>AETDVLIVGAGPAGAMSATLLASLGIRSLMINRWRSTSPGPRSHIINQRTMEILRDIGLEESAKSLAVPKEYMGEHVYATSLAGEEFGRIPAWASHPQAHAEHELASPSRYCDLPQLYFEPMVVSEAALRGADVRFLTEYLGHVEDQDGVTARLLDHVSGAEYEVRAKYIIGADGAHSLVAQNAGLPFEGQMGIGDSGSINIEFSADLSSLCEHRKGDMYWMFRAGSGINGVGVAALRMIRPWNKWICVWGYEKSKGTPEITKEEAKKIIHEIIGTDEIPVEVGPISTWTINQQYAVRNTSGRVFCMGDAVHRHTPAGGLGLNTSVQDAYNLAW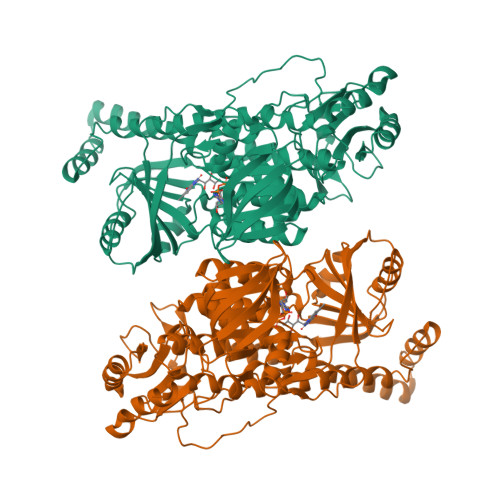KLALVLKGTAAPTLLDSYDAERSPVAKQIVERAFKSLSTFPPVFEALSLPPAPTESEMAEALVRLKDASEEGAKRRAALRKAMDATIIGLGGGHGVELNQRYVSRAVFPDGTPDPGFVRDQEFFYQASTRPGAHLPHVWLTENQRRISTLDLCGKGRFTLLTGLSGAAWKHEAEQVSQSLGIELKVCVIGPGQEFVDTYGEYAKISEIGESGALLVRPDMFIAFRAKDASREGLEQLNVAVKSILGR[2x]> DPIHDRTSDYHKYLKVKQGDSDLFKLTVSDKRYIWYNPDPKERDSYECGEIVSETSDSFTFKTVDGQDRQVKKDDANQRNPIKFDGVEDMSELSYLNEPAVFHNLRVRYNQDLIYTYSGLFLVAVNPFKIIPIYTQEMVDIFKGRRRNEVAPHIFAISDVAYRSMLDDRQNQSLLITGESGAGKTENTKKVIQYLASVAGRNQANGSGVLEQQILQANPILEAFGNAKTTRNNNSSRFGKFIEIQFNSAG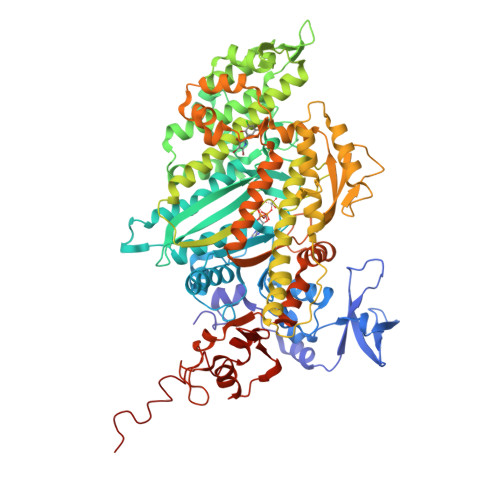FISGASIQSYLLEKSRVVFQSETERNYHIFYQLLAGATAEEKKALHLAGPESFNYLNQSGCVDIKGVSDSEEFKITRQAMDIVGFSQEEQMSIFKIIAGILHLGNIKFEKGAGEGAVLKDKTALNAASTVFGVNPSVLEKALMEPRILAGRDLVAQHLNVEKSSSSRDALVKALYGRLFLWLVIKINNVLCQERKAYFIGVLDISGFEIFKVNSFEQLCINYTNEKLQQFFNHHMFKLEQEEYLKEKINWTFIDFGLDSQATIDLIDGRQPPGILALLDEQSVFPNATDNTLITKLHSHFSKKNAKYEEPRFSKTEFGVTHYAGQVMYEIQDWLEKNKDPLQQDLELCFKDSSDNVVTKLFNDPNIASRAKKGANFITVAAQYKEQLASLMATLETTNPHFVRCIIPNNKQLPAKLEDKVVLDQLRCNGVLEGIRITRKGFPNRIIYADFVKRYYLLAPNVPRDAEDSQKATDAVLKHLNIDPEQYRFGITKIFFRAGQLARIEEAREQRLESNEPPMDFDDDIPF> ESDTGLWLHNKLGATDELWAPPSIASLLTAAVIDNIRLCFHGLSSAVKLKLLLGTLHLPRRTVDEMKGALMEIIQLASLDSDPWVLMVADILKSFPDTGSLNLELEEQNPNVQDILGELREKVGECEASAMLPLECQYLNKNALTTLAGPLTPPVKHFQLKRKPKSATLRAELLQKS;> GEITSVSTACQQLEVFSRVLRTSLATILDGGEENLEKNLPEFAKMVCHGEHTYLFAQAMMSVLAQEEQGGSAVRRIAQEVQRFAQEKGHDASQITLALGTAASYPRACQALGAMLSKGALNPADITVLFKMFTSMDPPPVELIRVPAFLDLFMQSLFKPGA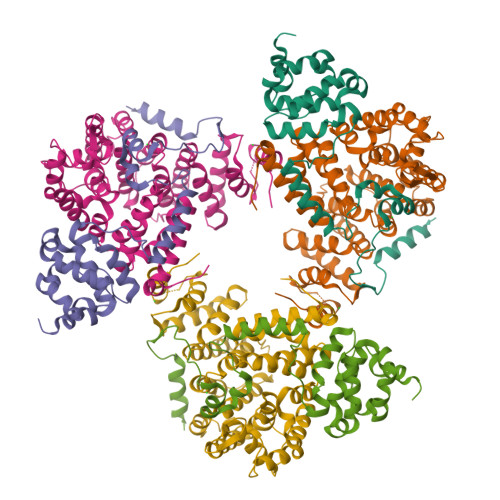RINQDHKHKYIHILAYAASVVETWKKNKRVSINKDELKSTSKAVETVHNLCCNENKGASELVAELSTLYQCIRFPVVAMGVLKWVDWTVSEPRYFQLQTDHTPVHLALLDEISTCHQLLHPQVLQLLVKLFETEHSALDVMEQLELKKTLLDRMVHLLSRGYVLPVVSYIRKCLEKLDTDISLIRYFVTEVLDVIAPPYTSDFVQLFLPILENDSIAGTIKTEGEHDPVTEFIAHCKSNFIMVN The P2X7 receptor is an ATP-gated ion channel that activates inflammatory pathways involved in diseases such as cancer, atherosclerosis, and neurodegeneration. When present in high concentrations, such as in pathological inflammatory states, extracellular ATP acts as a danger signal to cells by binding to and activating the P2X7 receptor (P2X7R). This spatiotemporal signaling stimulates the innate immune system by triggering assembly of the NLRP3 inflammasome and subsequent cytokine release, as well as activation of various less understood signaling cascades, ultimately resulting in apoptosis. P2X7R antagonists bind to either classical or extended allosteric ligand-binding sites that exist within the extracellular domain at the interface of two protomers.

To characterize the molecular differences between key mammalian P2X7R orthologs, we obtained cryo-EM structures of the full-length wild-type mP2X7 (2.5 Å) and hP2X7 (2.5 Å) receptors in the apo closed state conformation. However, we also identified ortholog-specific features in the hP2X7R, including two cholesterol hemisuccinate (CHS) binding sites per protomer at the interface between transmembrane helix 1 (TM1) and transmembrane helix 2 (TM2) on what would be the extracellular leaflet of the membrane bilayer. The two CHS molecules are stacked on top of each other such that the inner molecule is closer to the TM1/TM2 interface, and the outer molecule is positioned between TM1 and the inner molecule. The inner CHS molecule is coordinated by hydrophobic interactions with residues F328 and L333 on TM2; F38, V41, C42, L45, and Y51 on TM1; and W265 on the lower body domain. The outer CHS molecule is coordinated by hydrophobic interactions with residues F38, C42, and V46 on TM1; residue F266 on the lower body domain; and the inner CHS molecule. Interestingly, although not apparent from sequence alignments, our structure of the hP2X7R shows that the larger side chain of V312 forces the adjacent, conserved residue Y295 to adopt an alternative rotameric conformation compared to its conformation in both mP2X7R and rP2X7R, condensing the size of the pocket in hP2X7R. Thus, the classical allosteric ligand-binding site in the human ortholog has a different size and shape, which impacts the binding of allosteric antagonists. As a result of these residue differences, the classical allosteric pocket of the hP2X7R is smaller than in the rP2X7R or the mP2X7R in the apo closed state conformation. CHS-binding sites were only evident in the apo closed state structure of the hP2X7R. The CHS-binding sites are located on the extracellular leaflet of the membrane, similar to the location of CHS in the apo closed state structure of the hP2X1R and likely represent cholesterol binding sites in vivo.

>[3x]MPACCSCSDVFQYETNKVTRIQSMNYGTIKWFFHVIIFSYVCFALVSDKLYQRKEPVISSVHTKVKGIAEVKEEIVENGVKKLVHSVFDTADYTFPLQGNSFFVMTNFLKTEGQEQRLCPEYPTRRTLCSSDRGCKKGWMDPQSKGIQTGRCVVYEGNQKTCEVSAWCPIEAVEEAPRPALLNSAENFTVLIKNNIDFPGHNYTTRNILPGLNITCTFHKTQNPQCPIFRLGDIFRETGDNFSDVAIQGGIMGIEIYWDCNLDRWFHHCRPKYSFRRLDDKTTNVSLYPGYNFRYAKYYKENNVEKRTLIKVFGIRFDILVFGTGGKFDIIQLVVYIGSTLSYFGLAAVFIDFLIDTYSSNCCRSHIYPWCKCCQPCVVNEYYYRKKCESIVEPKPTLKYVSFVDESHIRMVNQQLLGRSLQDVKGQEVPRPAMDFTDLSRLPLALHDTPPIPGQPEEIQLLRKEATPRSRDSPVWCQCGSCLPSQLPESHRCLEELCCRKKPGACITTSELFRKLVLSRHVLQFLLLYQEPLLALDVDSTNSRLRHCAYRCYATWRFGSQDMADFAILPSCCRWRIRKEFPKSEGQYSGFKSPY>[8x]MGHHHHHHSGMKIAILGAMSEEITPLLETLKDYTKIEHANNTYYFAKYKD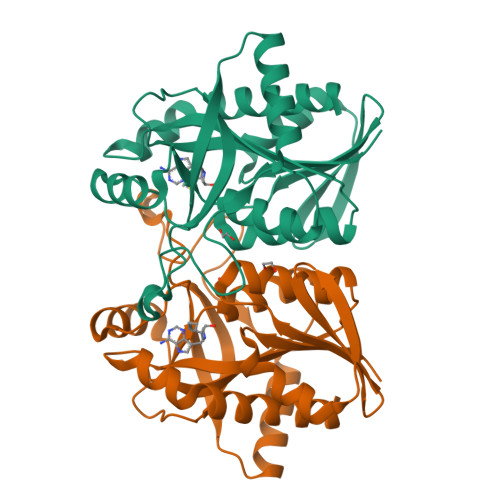HELVLAYSKIGKVNSTLSASVMIEKFGAQVLLFTGVAGAFNPELEIGDLLYATKLAQYDLDITAFGHPLGFVPGNEIFIKTDEKLNNLALEVAKELNIKLRAGIIATGDEFICDEAKKAKIREIFNADACEMEGASVALVCDALKVPCFILRAMSDKAGEKAEFDFDEFVINSAKISANFVLKMCEKL> GI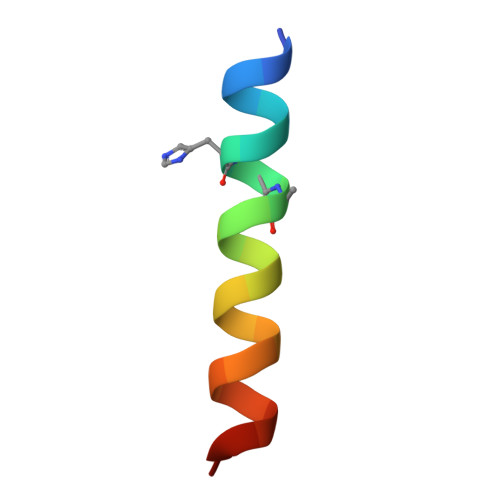GKFLHXAKKFAKAFVAEIMNS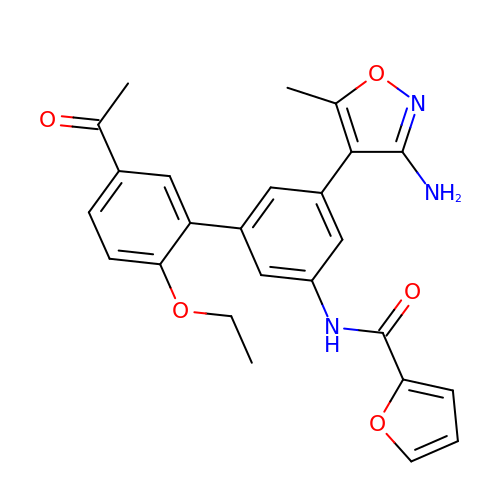~{N}-[3-(3-azanyl-5-methyl-1,2-oxazol-4-yl)-5-(5-ethanoyl-2-ethoxy-phenyl)phenyl]furan-2-carboxamide | C25 H23 N3 O5 | QBKCNTCHKRMYPR-UHFFFAOYSA-N> IWELKKDVYVVELDWYPDAPGEMVVLTCDTPEEDGITWTLDQSSEVLGSGKTLTIQVKEFGDAGQYTCHKGGEVLSHSLLLLHKKEDGIWSTDILKDQKEPKNKTFLRCEAKNYSGRFTCWWLTTISTDLTFSVKSSRGSSDPQGVTCGAATLSAERVRGDNKEYEYSVECQEDSACPAAEESLPIEVMVDAVHKLKYENYTSSFF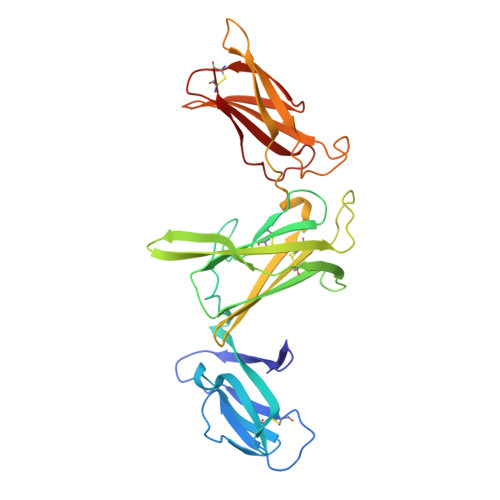IRDIIKPDPPKNLQLKPLKNSRQVEVSWEYPDTWSTPHSYFSLTFCVQVQGKSKREKKDRVFTDKTSATVICRKNASISVRAQDRYYSSSWSEWASVPCS>[2x]MMTLNRKCVVIHNGSHRTVAGFSNVELPQCIIPSSYIKRTDEGGEAEFIFGTYNMIDAAAEKRNGDEVYTLVDSQGLPYNWDALEMQWRYLYDTQLKVSPEELPLVITMPATNGKPDMAILERYYELAFDKLNVPVFQIVIEPLAIALSMGKSSAFVIDIGASGCNVTPIIDGIVVKNAVVRSKFGGDFLDFQVHERLAPLIKEENDMENMADEQKRSTDVWYEASTWIQQFKSTMLQVSEKDLFELERYYKEQADIYAKQQEQLKQMDQQLQYTALTGSPNNPLVQKKNFLFKPLNKTLTLDLKECYQFAEYLFKPQLISDKFSPEDGLGPLMAKSVKKAGASINSMKANTSTNPNGLGTSHINTNVGDNNSTASSSNISPEQVYSLLLTNVIITGSTSLIEGMEQRIIKELSIRFPQYKLTTFANQVMMDRKIQGWLGALTMANLPSWSLGKWYSKEDYETLKRDRKQSQATNATNLV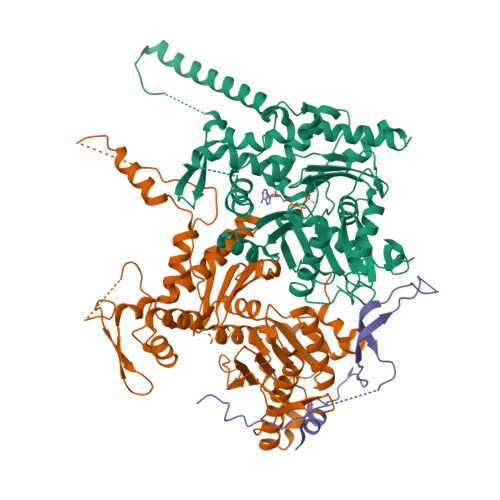PRGSHHHHHH;>MAPFRQDSILIIYPRSQTTLVQFGLNEETFTVPELEIPTQIYRTTRQDGSYTYHSTNKDNKAELIKPIQNGEIIDISAFTQFLRLIFVSILSDRANKNQDAFEAELSNIPLLLITHHSWSQSDLEIITQYVFESLEINNLIQLPASLAATYSMISLQNCCIIDVGTHHTDIIPIVDYAQLDHLVSSIPMGGQSINDSLKKLLPQWDDDQIESLKKSPIFEVLSDDAKKLSSFDFGNENEDEDEGTLNVAEIITSGRDTREVLEERERGQKVKNVKNSDLEFNTFWDEKGNEIKVGKQRFQGCNNLIKNISNRVGLTLDNIDDINKAKAVWENIIIVGGTTSISGFKEALLGQLLKDHLIIEPEEEKSKREEEAKSVLPAATKKKSKFMTNSTAFVPTIEYVQCPTVIKLAKYPDYFPEWKKSGYSEIIFLGAQIVSKQIFTHPKDTFYITREKYNMKGPAALWDVQF[2x];>[2x]SMDPQTLITKANKVSYYGNPTSKESWRYDWYQPSKVSSNVQQPQQQLGDMENNLEKYPFRYKTWLRNQEDEKNLQRESCEDILDLKEFDRRILKKSLMTSHTKGDTSKATGAPSANQGDEALSVDDIRGAVGNSEAIPGLSAGVNNDNTKESKDVKMN MAG is a type 1 single-pass transmembrane protein expressed on myelinating oligodendrocytes in the CNS and Schwann cells in the PNS23. Myelin-associated glycoprotein (MAG) adhesion and signalling at the myelin–axon interface regulates the formation and maintenance of myelinated axons, thus playing an important role in the development and function of the nervous system. MAG adhesion maintains the myelin–axon spacing (periaxonal diameter) by interacting with specific neuronal gangliosides (glycolipids), such as the major brain gangliosides GT1b and GD1a. On the basis of the primary sequence its extracellular region is predicted to consist of five Ig domains; an N-terminal V-type Ig domain that is typical for Siglecs and four C2-type Ig domains.

To obtain more detailed information on MAG–ligand interactions, the commercially available trisaccharide 3′-N-Acetylneuraminyl-N-acetyllactosamine (Neu5Ac-α2,3-Gal-β1,4-GlcNAc) was soaked into the MAG1–3 crystals, as these provided higher resolution data. For the soaked crystals, diffraction data was collected to 2.3 Å resolution. The crystals were isomorphous to the unsoaked MAG1–3 crystals and a Fo(soaked)−Fo(unsoaked) map revealed clear electron density in the oligosaccharide binding site for one of the two MAG1–3 chains in the asymmetric unit. Most likely the other chain remained unliganded due to occlusion of the binding site by crystal packing. The ganglioside binding side is formed by the CC′ loop and the F and G β-strands of the N-terminal V-type Ig1 domain. In agreement with previous data, the side chain of R118 in strand F forms a key salt bridge with the carboxylic acid group of the sialic acid in the trisaccharide ligand. Y65 in the CC′ loop forms extensive Van der Waals' contacts with the ligand as well as a hydrogen bond to the O9 of the Neu5Ac sialic acid. Other contributing interactions are made by: (1) the backbone carbonyls of N126 and T128 in strand G that form hydrogen bonds with H-N5 and the H-O9 of the sialic acid respectively, (2) the backbone amide proton of T128 that forms a hydrogen bond with the O8 of the sialic acid and (3) the side chain of Y127 that forms Van der Waals' contacts with the glycerol group (C7–C9) of the sialic acid. Ligand interaction of MAG is similar to the sialic acid recognition of other Siglec family members.

>[2x]GSGHWGAWMPSTISAFEGTCVSIPCRFDFPDELRPAVVHGVWYFNSPYPKNYPPVVFKSRTQVVHESFQGRSRLLGDLGLRNCTLLLSTLSPELGGKYYFRGDLGGYNQYTFSEHSVLDIVNTPNIVVPPEVVAGTEVEVSCMVPDNCPELRPELSWLGHEGLGEPTVLGRLREDEGTWVQVSLLHFVPTREANGHRLGCQAAFPNTTLQFEGYASLDVKYPPVIVEMNSSVEAIEGSHVSLLCGADSNPPPLLTWMRDGMVLREAVAKSLYLDLEEVTPGEDGVYACLAENAYGQDNRTVELSVMYAAAAHHHHHH>MADDAIPHTDVLNSTAQGQLKSIIERVERLEVEKAEIMEQIKEVYAEAKGNG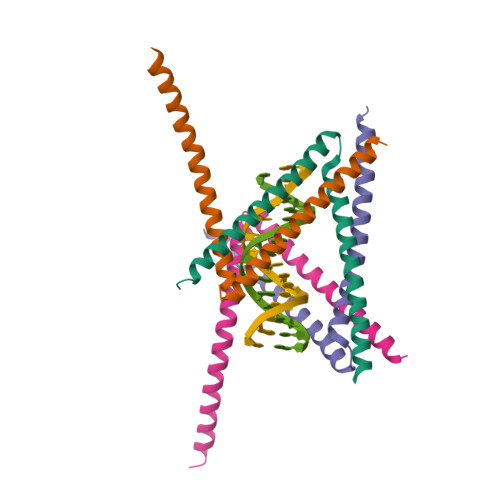FDVKVLKKVVRIRKQDRAKRQEEDAILDLYLSAIGEILEHHHHHH[4x]>[12x]MNYETLLPLQTIREHAKCDDNPRVTDTLLSLYREAAFEAAELYTGMSFTPQKTIVEPVRIK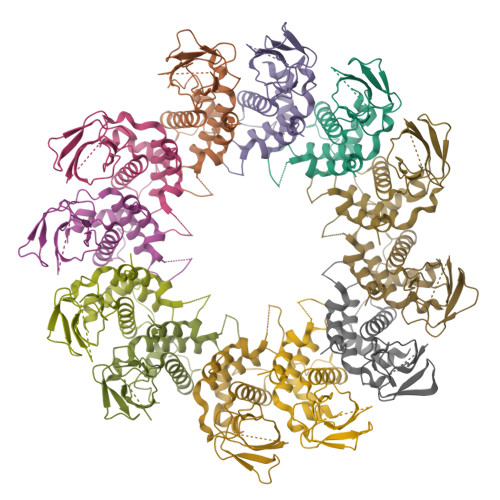NRKGKIVLSQVPIAGRPVVFTGGGLGSPLELIPFPNSNVLHFPNGSPDRFQTWGDCHTCGVPSQLMATYVAGRRCESSVPAGIIMGVLKLIAWNINNPGDEIMSVRNTSTANAQGLIGGTNNGAVVSGAQDEWFRYRRVIL> MNLMTTITGVVLAGGKARRMGGVDKGLLELNGKPLWQHVADALMTQLS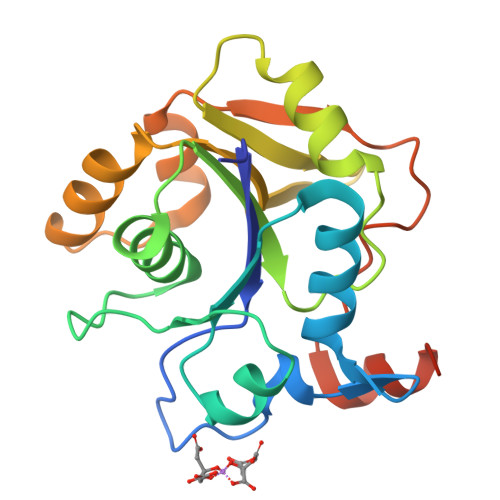HVVVNANRHQEIYQASGLKVIEDSLADYPGPLAGMLSVMQQEAGEWFLFCPCDTPYIPPDLAARLNHQRKDAPVVWVHDGERDHPTIALVNRAIEPLLLEYLQAGERRVMVFMRLAGGHAVDFSDHKDAFVNVDTPEELARWQEKRSHHHHHH>[2x]MSTQYETQGYTINNAGRRLVVDPITRIQGHMRCEVNINDQNVITNAVSCGTMFRGLEIILQGRDPRDAWAFVERICGVCTGVHALASVYAIEDAIGIKVPDNANIIRNIMLATLWCHDHLVHFYQLAGMDWIDVLDALKADPRKTSELAQSLSSWPKSSPGYFFDVQNRLKKFVEGGQLGIFRNGYWGHPQYKLPPEANLMGFAHYLEALDFQREIVKIHAVFGGKNPHPNWIVGGMPCAINIDESGAVGAVNMERLNLVQSIITRTADFINNVMIPDALAIGQFNKPWSEIGTGLSDKCVLSYGAFPDIANDFGEKSLLMPGGAVINGDFNNVLPVDLVDPQQVQEFVDHAWYRYPNDQVGRHPFDGITDPWYNPGDV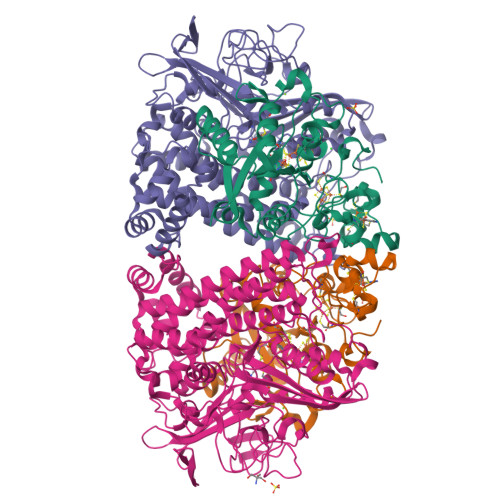KGSDTNIQQLNEQERYSWIKAPRWRGNAMEVGPLARTLIAYHKGDAATVESVDRMMSALNLPLSGIQSTLGRILCRAHEAQWAAGKLQYFFDKLMTNLKNGNLATASTEKWEPATWPTECRGVGFTEAPRGALGHWAAIRDGKIDLYQCVVPTTWNASPRDPKGQIGAYEAALMNTKMAIPEQPLEILRTLHSFDPCLACSTH;>LENKPRIPVVWIHGLECTCCTESFIRSAHPLAKDVILSLISLDYDDTLMAAAGTQAEEVFEDIITQYNGKYILAVEGNPPLGEQGMFCISSGRPFIEKLKRAAAGASAIIAWGTCASWGCVQAARPNPTQATPIDKVITDKPIIKVPGCPPIPDVMSAIITYMVTFDRLPDVDRMGRPLMFYGQRIHDKCYRRAHFDAGEFVQSWDDDAARKGYCLYKMGCKGPTTYNACSSTRWNDGVSFPIQSGHGCLGCAENGFWDRGSFYSRVVDIPQMGTHSTADTVGLTALGVVAAAVGVHAVASAVDQRRRHNQQPTETEHQPGNEDKQARSHHHHHH[2x]> MNYTETVAYIHSFPRLAKTGDHRRILTLLHALGNPQQQGRYIHVTGTNGKSTAANAIAHVLEASGLTVGLYTSPFIMRFNERIMIDHEPIPDAALVNAVAFVRAALERLQQQQA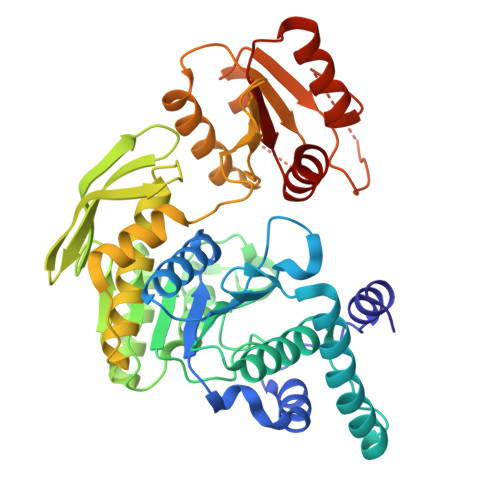DFNVTEFEFITALGYWYFRQRQVDVAVIEVGIGGDTDSTNVITPVVSVLTSVALDHQKLLGHTITAIAKHKAGIIKRGIPVVTGNLVPDAAAVVAAKVATTGSQWLRFDRDFSVPKAKLHGWGQRFTYEDQDGRISDLEVPLVGDYQQRNMAIAIQTAKVYAKQTEWPLTPQNIRQGLAASHWPARLEKISDTPLIVIDGAHNPDGINGLITALKQLFSQPITVIAGILADKDYAAMADRLTAAFSTVYLVPVPGTPRALPEAGYEALHEGRLKDSWQEALAASLNDVPDQPIVITGSLYLASAVRQTLLGGKS>[2x]MKHSLPDLPYDYADLEPVISHEIMQLHHQKHHATYVNNLNQIEEKLHEAVSKGNVKEAIALQPA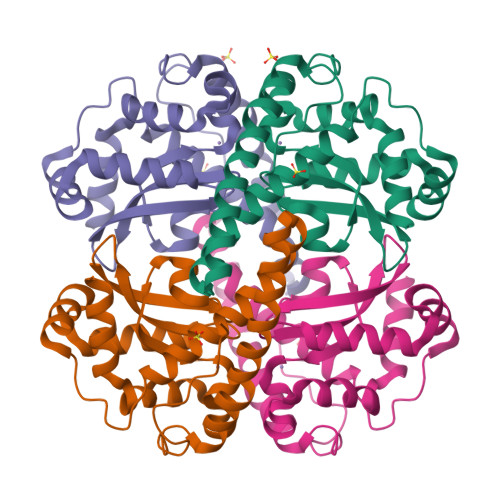LKFNGGGHINHSIFWTNLAKDGGEPSAELLTAIKSDFGSLDNLQKQLSASTVAVQGSGWGWLGYCPKGKILKVATCANQDPLEATTGLVPLFGIDVWEHAYYLQYKNVRPDYVNAIWKIANWKNVSERFAKAQQ>MIKRYDVAEISKIWADENKYAKMLEVELAILEALEDRMVPKGTAAEIRARAQIRPERVDEIEKVTKHDIIAFCTSIAEQFTAETGKFFHFGVTSSDIIDSALSLQIRDSMSYVIKDLEALCDSLLTKAEETKEIITMGRSHGMFAEPMSFGQKFLGAYVEFKRRLKDLKDFQKDGLTVQFSGAVGNYCILTTEDEKKAADILGLPVEEVS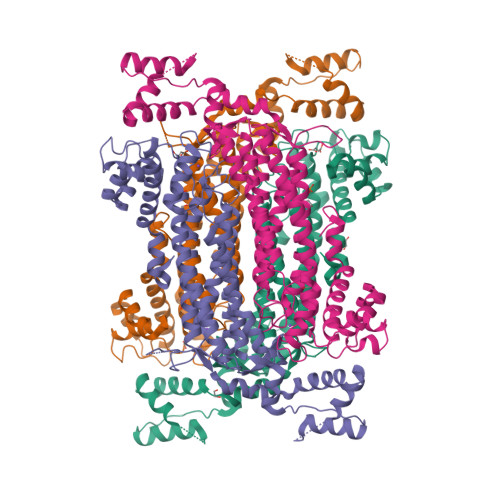TQVIPRDRIAKLISIHGLIASAIERLAVEIRHLHRSDVFEVYEGFSKGQKGSSTMPHKKNPISTENLTGMARMLRSHVSIALENCVLWHERDISHSSAERFYLPDNFGIMVYALRRMKNTIDNLVVQRDIIEDRVRSTSAYLSSFYLHFLVANTPFMREDCYKIVQQVAFDLKQGESFSKKLQKVMHDEHNIILDIPEMDFEGIKKTYLKEIDHVFDRSVKARGENLY[4x]>MGHHHHHHAENLYFQGHMHK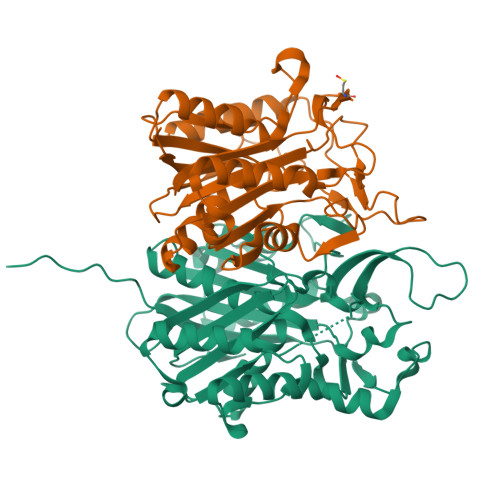VKLAAITCELPARSYENDDPVFAAVPDLSESWWQFWGVNRRGYFDPRNGENEFSLVVRAAERLLRSSDTAPDSVDMLICSASSPIMTDAGDVLPDLRGRLYPRMANVLSKQLGLSRALPLDSQMECASFLLNLRLAASMIRQGKAEKVLVVCSEYISNLLDFTSRTSTLFADGCAVALLTRGDDDSCDLLASAEHSDATFYEVATGRWRLPENPTGEAKPRLYFSLFSDGQNKMASFVPTNVPIAMRRALEKAGLGSDDIDYFVFHQPAPFLVKAWAEGIGARPEQYQLTMGDTGVMISVSIPYTLMTGLREGKIRPGDRIVMAGAATGWGFAAQVWQLGEVLVC[4x];>[4x]MLIQAVGVNLPPSYVCLEGPLGGERPRAQGDEMLMQRLLPAVREALDEAAVKPEEIDLIVGLALSPDHLIENRDIMAPKIGHPLQKVLGANRAHVFDLTDSSLARALYVVDTLASDQGYRNVLVVRGESSQGLEVDSESGFALADGALALLCRPTGKAAFRRGALGGDPAQEWLPLSIPLNTDIRQVGDVKGHLNLPAQPGLPEAVRAGFTRLAGDFPQLNWVREEWFGQGRPDGRCLGPFELASQLRAAQRDRLDELLLISFDPFGMVVEGVTLELAGEAHA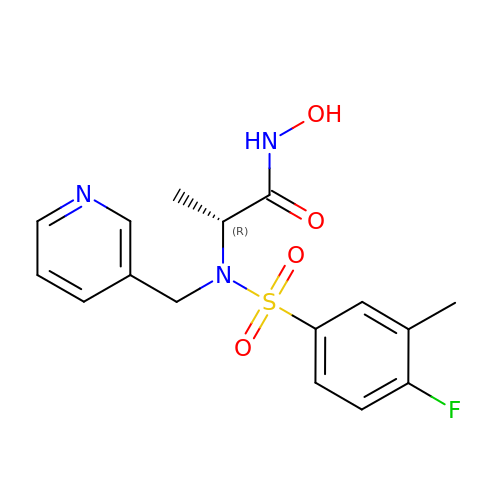N~2~-[(4-fluoro-3-methylphenyl)sulfonyl]-N-hydroxy-N~2~-(pyridin-3-ylmethyl)-D-alaninamide | C16 H18 F N3 O4 S | OFKSJKLKSOBXCJ-GFCCVEGCSA-N>[2x]MEVSPLQPVNENMQVNKIKKNEDAKKRLSVERIYQKKTQLEHILLRPDTYIGSVELVTQQMWVYDEDVGINYREVTFVPGLYKIFDEILVNAADNKQRDPKMSCIRVTIDPENNLISIWNNGKGIPVVEHKVEKMYVPALIFGQLLTSSNYDDDEKKVTGGRNGYGAKLCNIFSTKFTVETASREYKKMFKQTWMDNMGRAGEMELKPFNGEDYTCITFQPDLSKFKMQSLDKDIVALMVRRAYDIAGSTKDVKV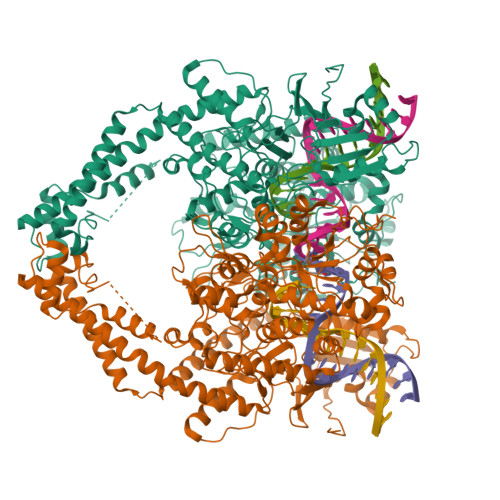FLNGNKLPVKGFRSYVDMYLKDKLDETGNSLKVIHEQVNHRWEVCLTMSEKGFQQISFVNSIATSKGGRHVDYVADQIVTKLVDVVKKKNKGGVAVKAHQVKNHMWIFVNALIENPTFDSQTKENMTLQPKSFGSTCQLSEKFIKAAIGCGIVESILNWVKFKAQVQLNKKCSAVKHNRIKGIPKLDDANDAGGRNSTECTLILTEGDSAKTLAVSGLGVVGRDKYGVFPLRGKILNVREASHKQIMENAEINNIIKIVGLQYKKNYEDEDSLKTLRYGKIMIMTDQDQDGSHIKGLLINFIHHNWPSLLRHRFLEEFITPIVKVSKNKQEMAFYSLPEFEEWKSSTPNHKKWKVKYYKGLGTSTSKEAKEYFADMKRHRIQFKYSGPEDDAAISLAFSKKQIDDRKEWLTNFMEDRRQRKLLGLPEDYLYGQTTTYLTYNDFINKELILFSNSDNERSIPSMVDGLKPGQRKVLFTCFKRNDKREVKVAQLAGSVAEMSSYHHGEMSLMMTIINLAQNFVGSNNLNLLQPIGQFGTRLHGGKDSASPRYIFTMLSSLARLLFPPKDDHTLKFLYDDNQRVEPEWYIPIIPMVLINGAEGIGTGWSCKIPNFDVREIVNNIRRLMDGEEPLPMLPSYKNFKGTIEELAPNQYVISGEVAILNSTTIEISELPVRTWTQTYKEQVLEPMLNGTEKTPPLITDYREYHTDTTVKFVVKMTEEKLAEAERVGLHKVFKLQTSLTCNSMVLFDHVGCLKKYDTVLDILRDFFELRLKYYGLRKEWLLGMLGAESAKLNNQARFILEKIDGKIIIENKPKKELIKVLIQRGYDSDPVKAWKEAQQKVPDEEENEESDNEKETEKSDSVTDSGPTFNYLLDMPLWYLTKEKKDELCRLRNEKEQELDTLKRKSPSDLWKEDLATFIEELEAVEAKEKQDEQVGLPGKGGKAKGKKTQMAEVLPSPRGQRVIPRITIEMKAEAEKKNKKKIKNENTEGSPQEDGVELEGLKQRLEKKQKREPGTKTKKQTTLAFKPIKKGKKRNPWSDSESDRSSDESNFDVPPRETEPRRAATKTKFTMDLDSDEDFSDFDEKTDDEDFVPSDASPPKTKTSPKLSNKELKPQKSVVSDLEADDVKGSVPLSSSPPATHFPDETEITNPVPKKNVTVKKTAAKSQSSTSTTGAKKRAAPKGTKRDPALNSGVSQKPDPAKTKNRRKRKPSTSDDSDSNFEKIVSKAVTSKKSKGESDDFHMDFDSAVAPRAKSVRAKKPIKYLEESDEDDLF>[2x]NVEEETKYIELMIVNDHLMFKKHRLSVVHTNTYAKSVVNMADLIYKDQLKTRIVLVAMETWATDNKFAISENPLITLREFMKYRRDFIKEKSDAVHLFSGSQFESSRSGAAYIGGICSLLKGGGVNEFGKTDLMAVTLAQSLAHNIGIISDKRKLASGECKCEDTWSGCIMGDTGYYLPKKFTQCNIE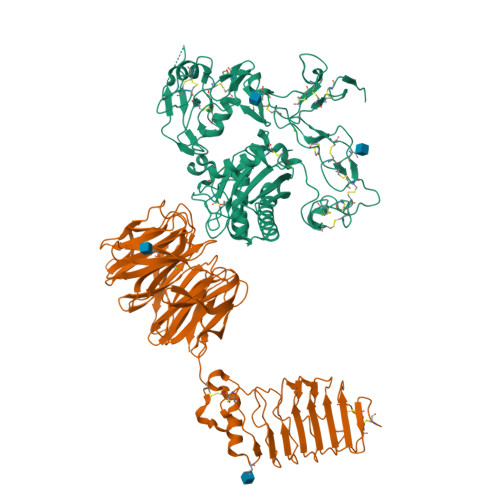EYHDFLNSGGGACLFNKPSKLLDPPECGNGFIETGEECDCGTPAECVLEGAECCKKCTLTQDSQCSDGLCCKKCKFQPMGTVCREAVNDCDIRETCSGNSSQCAPNIHKMDGYSCDGVQGICFGGRCKTRDRQCKYIWGQKVTASDKYCYEKLNIEGTEKGNCGKDKDTWIQCNKRDVLCGYLLCTNIGNIPRLGELDGEITSTLVVQQGRTLNCSGGHVKLEEDVDLGYVEDGTPCGPQMMCLEHRCLPVASFNFSTCLSSKEGTICSGNGVCSNELKCVCNRHWIGSDCNTYFPHNDDAKTGITLSG;>DAAQPARRARRTYEAYPAKPKCPAVCTCTKDNALCENARSIPRTVPPDVISLSFVRSGFTEISEGSFLFTPSLQLLLFTSNSFDVISDDAFIGLPHLEYLFIENNNIKSISRHTFRGLKSLIHLSLANNNLQTLPKDIFKGLDSLTNVDLRGNSFNCDCKLKWLVEWLGHTNATVEDIYCEGPPEYKKRKINSLSSKDFDCIITEFAKSQDLPYQSLSIDTFSYLNDEYVVIAQPFTGKCIFLEWDHVEKTFRNYDNITGTSTVVCKPIVIETQLYVIVAQLFGGSHIYKRDSFANKFIKIQDIEILKIRKPNDIETFKIENNWYFVVADSSKAGFTTIYKWNGNGFYSHQSLHAWYRDTDVEYLEIVRTPQTLRTPHLILSSSSQRPVIYQWNKATQLFTNQTDIPNMEDVYAVKHFSVKGDVYICLTRFIGDSKVMKWGGSSFQDIQAMPSRGSMVFQPLQINNYQYAILGSDYSFTQVYNWDAEKAKFVKFQELNVQAPRSFTHVSINKRNFLFASSFKGNTQIYKHVIVDLSAKHHHHHH[2x]> MTRINLTLVSELADQHLMAEYRDLPRV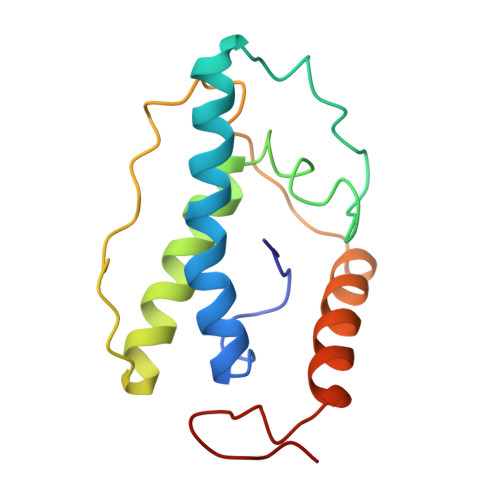FGAVRKHVANGKRVRDFKISPTFILGAGHVTFFYDKLEFLRKRQIELIAECLKRGFNIKDTTVQDISDIPQEFRGDYIPHEASIAISQARLDEKIAQRPTWYKYYGKAIYA> CLTAPPKEAARPTLMPRAQSYKDLTHLPAPTGKIFVSVYNIQDETGQFKPYPASNFSTAVPQSATAMLVTALK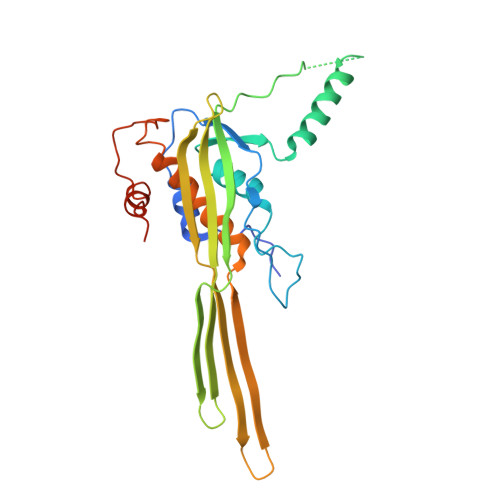DSRWFIPLERQGLQNLLNERKIIRAAQENGTVAINNRIPLQSLTAANIMVEGSIIGYESNVKSGGVGARYFGIGADTQYQLDQIAVNLRVVNVSTGEILSSVNTSKTILSYEVQAGVFRFIDYQRLLEGEVGYTSNEPVMLCLMSAIETGVIFLINDGIDRGLWDLQNKAERQNDILVKYRHMSVPPESSAWSHPQFEK> MYVYKRDGRKEPVQFDKITARISRLCYGLDPKHIDAVKVTQRIISGVYEGVTTIELDNLAAETCAYMTTVHPDYATLAARIAISNLHKQTTKQFSKVVEDLYRYVNAATGKPAPMISDDVYNIVMENKDKLNSAIVYDRDFQYSYFGFKTLERSYLLRINGQVAERPQHLIMRVALGIHGRDIEAALETYNLMSLKYFTHASPTLFNAGTPKPQMSSCFLVAMKEDSIEGIYDTLKECALISKTAGGIGLHIHNIRSTGSYIAGTNGTSNGLIPMIRVFNNTAR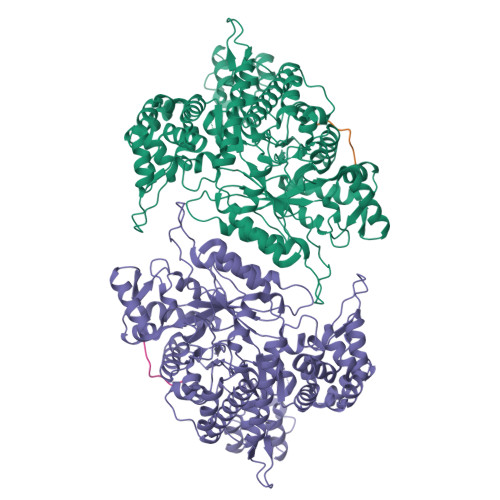YVDQGGNKRPGAFALYLEPWHADIFDFIDIRKNHGKEEIRARDLFPALWIPDLFMKRVEENGTWTLFSPTSAPGLSDCYGDEFEALYTRYEKEGRGKTIKAQKLWYSILEAQTETGTPFVVYKDACNRKSNQKNLGVIKSSNLCCEIVEYSAPDETAVCNLASVALPAFIETSEDGKTSTYNFKKLHEIAKVVTRNLNRVIDRNYYPVEEARKSNMRHRPIALGVQGLADTFMLLRLPFDSEEARLLNIQIFETIYHASMEASCELAQKDGPYETFQGSPASQGILQFDMWDQKPYGMWDWDTLRKDIMKHGVRNSLTMAPMPTASTSQILGYNECFEPVTSNMYSRRVLSGEFQVVNPYLLRDLVDLGIWDEGMKQYLITQNGSIQGLPNVPQELKDLYKTVWEISQKTIINMAADRSVYIDQSHSLNLFLRAPTMGKLTSMHFYGWKKGLKTGMYYLRTQAASAAIQFTIDQKIADQATENVADISNLKRPSYMPSSASYAASDFVPAAVTANATIPSLDSSSEASREASPAPTGSHSLTKGMAELNVQESKVEVPEVPAPTKNEEKAAPIVDDEETEFDIYNSKVIACAIDNPEACEMCSG;> FTLDADF>QIIGTVPGVEVGDEFQYRMELNLLGIHRPSQSGIDYMKDDGGELVATSIVSSGGYNDVLDNSDVLIYTGQGGNVGKKKNNEPPKDQQLVTGNLALKNSIN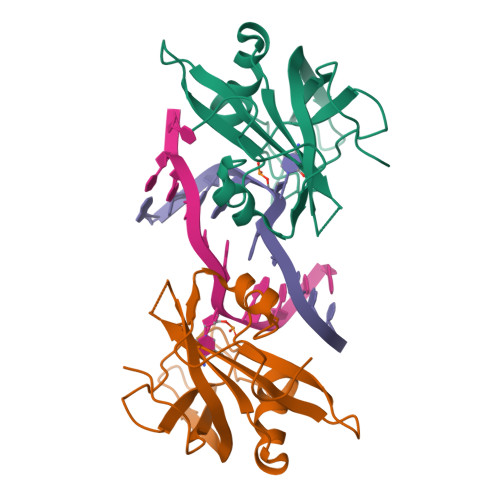KKNPVRVIRGIKNTTLQSSVVAKNYVYDGLYLVEEYWEETGSHGKLVFKFKLRRIPGQPELPWKEVA[2x]> MSMTEFTLLRWLREGRQSRKLILLIVFIALLLDNMLLTVVVPIIPSYLYSMTHESNNTHDGSIPPAAPSGFHSIFSYYDNTTVITTNFTSSDQLQQSALTPTTSPSLATPPASADCPKADSSLLNENVKVGLLFASKATVQLLTNPFIGPMTNRIGYQIPMFAGFCIMFVSTIMFAFSGTYTLLFIARSLQGIGSSCSSVAGMGMLASVYTDDEERGNAMGVALGGLAMGVLVGPPFGSILYEFVGKTAPFIVLAVLVLFDGALQLFVLQPSRVQPESQTGTPLLTLIRDPYILI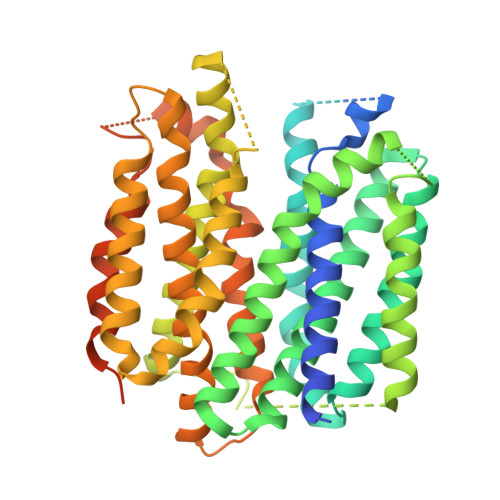AAGSICFANMAIAMLEPALPIWMMETMCSRKWQLGVAFLPASISYLLGTNIFGPLAHKMGRWLCAFIGMIMVGISIICVPFARNIYGLIAPNFGVGFAIGMVDSSMMPIMGYLVDLRHVSVYGSVYAIADVAFCMGFAFGPSAGGAIAKSIGFPWLMTIIGVVDILFAPLCLFLRSPPAREEKMAILMDHKCPVKTKMYTQNSGQPYYTGEEEESESDE> GSKRFSDIPQTIDIPMQDDVEVEIDLQVLPDDPTELCSVFENEQSPRIYWMTVALAYAKQNKIDFAIEMLLRGANVLQGNQREKLGIITCICWLYLWKSREAPRVAPDGVPASEAKTKEYYLQLATQSLNDASRINPAFPPLFLARGVLILLKASLQPSSKAPGAVDSNKAEQLRNALKSFEEAIRVSQGRNMLAVMGKARALFSLGRYPESLAAYQDVVAKMPDMVDPDPRIGIGCCFWQLGFKDDAKIAWERCLEINPDSKHANILLGLYYLDASGHVPTNSP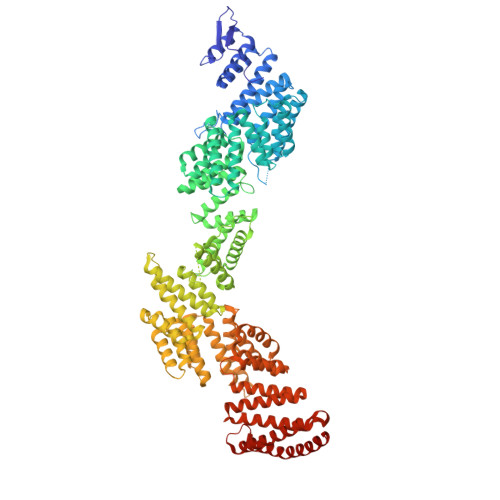EFIRLYKKAMTEYTQKSFKLDKNLPLTCATFAGYFLSRKQFGNVDALAHKAIQYTDVNAIASDGWYLLARKEHYDGNLERASDYYRRADDARGGAERGYLPAKFGAAQLSVLKNDLGEAKLRLEKMIQHSKNYEAMILLGTLYAEEVFANQSAAVKEDKSAEAKKAISLLEGVRSAWKDPKRNLSPDAAVLLNLARLYESESPDKALQCLQQVEQLEIDQIPQSEYPPDAEDEAAARAAIRKLLPPQLLNNIGCFYSQEGKHRLATEFFQAALDSCARISQTENDLDIDALLTTIPFNLGRSYEYEGDIDKAIETYEQLLSRHSDYTDARTRLAYIKLRRNPNKEGPDAVAKLYQENPSDLEVRGLYGWFLSKVNSKKRPANIAEDPEQRHYKHTLQSYDKHDRYALVGMGNLHLMAAREMRRETEQDRQKRSAAYNRAVEFFDKALQLDPKNAYAAQGIAIALVEDRKDYKNALQIFIKVRETIQDAHVYVNMGHIYAELRQFSKAIESYEIALSKEGKANDAGIISCLGRTWLNKGRAERNLDAYKMALDQAKKAVAVAPDQLHFKFNVAFVQIQIALVLHSMRESERNSFQLEEAAEGLEEAIKILDEIAASPSPPYPRHDIEQRANMARNTQRKQLERALASQREYEAKN>NAMPIEIITDSGADLPQSYIREHRIAFLPLVVHWNGQDYKDGITIEPKQVYDAMRQGHTVKTAQPSPLAMKELFLPYAKENRPCLYIAFSSKLSGTYQTAMAVRSELLDEYPEFRLTIIDSKCASLGQGLAVMKAVELAKQNTPYNLLCETIESYCRHMEHIFTVDNLDYLARGGRISKTAAAFGGLLNIKPLLHVEDGALIPLEKWRGRKKVLKRMVELMGERGDDLQKQTIGISHADDEETALELKQMIEETHGCTRFFLSDIGSAIGAHAGPGTIALFFLNKYIEI[2x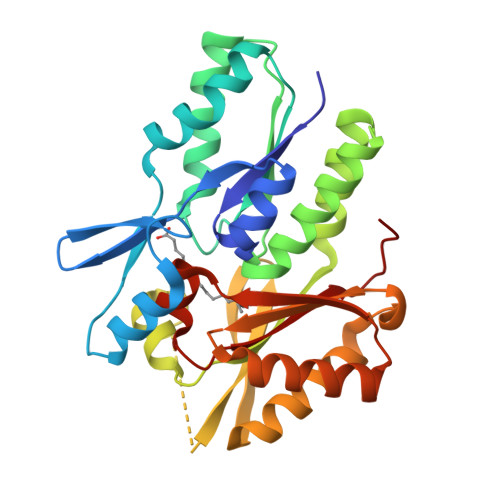]(2R,3R,4R,5R,6R)-5-acetamido-6-[(1R)-1,3-bis(oxidanyl)propyl]-2,3-bis(fluoranyl)-4-oxidanyl-oxane-2-carboxylic acid | C11 H17 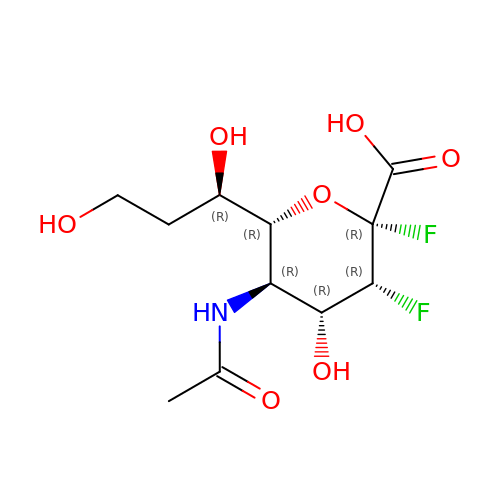F2 N O7 | SVILRGMXTMNWJP-XYLHZXCYSA-N> MGNPMNTTQLGKSLFQWQVEQEESKLANISQDQFLSKDADGDTFLHIAVAQGRRALSYVLARKMNALHMLDIKEHNGQSAFQVAVAANQHLIVQDLVNIGAQVNTTDCWGRTPLHVCAEKGHSQVLQAIQKGAVGSNQFVDLEATNYDGLTPLHCAVIAHNAVVHELQRNQQPHSPEVQELLLKNKSLVDTIKCLIQMGAAVEAKDRKSGRTALHLAAEEANLELIRLFLELPSCLSFVNAKAYNGNTALHVAASLQYRLTQLDAVRLLMRKGADPSTRNLENEQPVHLVPDGPVGEQIRRILKGKSIQQRAPPY;>ASNLKIVRMDRTAGCVTGGEEIYLLCDKVQKDDIQIRFYEEEENGGVWEGFGDFSPTDVHRQFAIVFKTPKYKDVNITKPASVFVQ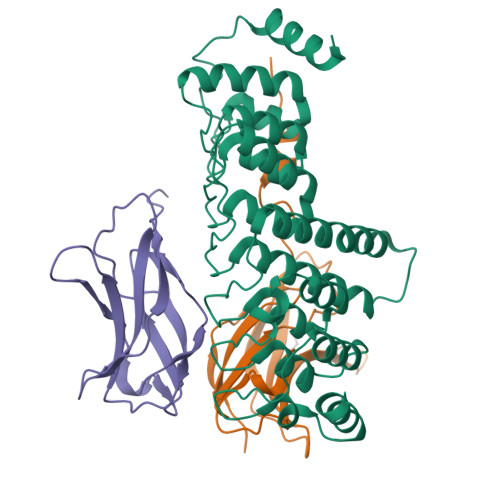LRRKSDLETSEPKPFLYYPEIKDKEEVQRKRQKLMPNFSDSFGGGS[2x]>[3x]M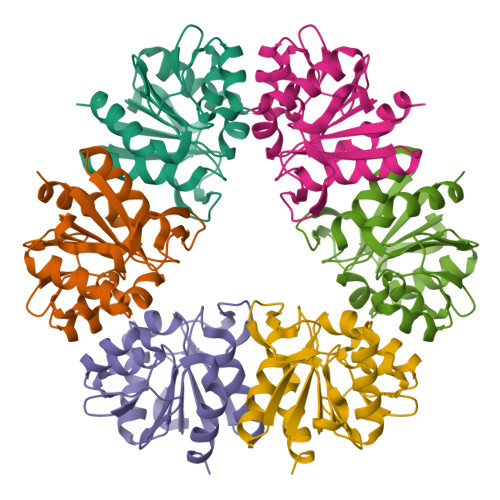KVLFLTANEFEDVELIYPYHRLKEEGHAVYIASFERGTITGKHGYSVKVDLTFDKVNPAEFDALVLPGGRAPERVRLNAKAVSIARKMFSEGKPVASICHGPQILISAGVLRGRKGTSYPGIKDDMINAGVEWVDAEVVVDGNWVSSRVPADLYAWMREFVKLLK> GPPYCVFPGRRTSSTSFTTSFSTEPLGYARMLHRDPPYERAGNSGLNHRIYERSRVGGLRTVIDVAPPDGHQAIANYEIEVRRIPVATPNAAGDCFHTARLSTGSRGPATISWDADASYTYYLTISED

Fusarium oxysporum f. sp. lycopersici (Fol), the causal agent of tomato wilt disease, produces effector protein Avr2. Avr2 is required for Fol virulence in susceptible tomato varieties, but triggers resistance in plants carrying I‐2 (Houterman et al., 2009). The Avr2 protein is recognized by I‐2 inside the plant nucleus (Ma et al., 2013) and exerts its virulence function inside host cells (Di et al., 2016). Consistent with the potential for Avr2 to target a conserved defense mechanism in different hosts, we demonstrate that Avr2 suppresses PRR (FLS2)‐mediated responses, such as growth inhibition, ROS production, MAPK activation and callose deposition following flagellin22 (flg22) treatment.

In an attempt to resolve the structural requirements underlying I‐2‐mediated recognition of Avr2, and its relationship to virulence, we determined the crystal structure of this effector. Structural homology searches revealed that Avr2 shares an overall β‐sandwich fold with the Pyrenophora tritici‐repentis effector ToxA and TRAF‐domain containing proteins, despite sharing no identifiable sequence similarity (no difference from chance). Given the lack of sequence identity, concluding that Avr2 shares a specific function with Tumor necrosis factor Receptor Associated Factor (TRAF)‐domain containing proteins (such as interfering with host ubiquitin ligase activity) is not possible. However, it is tempting to speculate that Avr2, in having this protein fold, may function (like other TRAFs) as an adapter unit, competing with host factors for target binding or binding to a host target and modulating its function. The crystal structure of Avr2 has revealed that Fol race 3 variants Avr2V41M, Avr2R45H, Avr2R46P and Avr2T50− are all within surface‐exposed residues that cluster on a loop, forming a distinct epitope. Notably, the residues that form this epitope are anchored in position by Cys40 forming a disulphide bound at one end (the far N‐terminus), and at the start of β1 (residue Ser51). Such an anchored extension is not observed in ToxA or other TRAF‐like proteins. We predict that molecular interactions involving this region are critical for I‐2‐mediated recognition and underlie the ability of the Fol race 3 variants to evade this. Our screen identified two threonine residues in Avr2 (Avr2T53 and Avr2T145) that are required for virulence (suppression of PTI), but not for I‐2‐mediated recognition. Avr2T145 is positioned within a putative functional site identified from comparison with the ligand‐bound structures of Speckle‐type POZ (SPOP) protein and TRAF6, and Avr2T53 is positioned within a putative functional site identified from comparison with the ligand‐bound structure of SIAH1.4,4'-(1-PROPYL-1H-1,2,4-TRIAZOLE-3,5-DIYL)BIS(2,5-DIHYDRO-1,2,5-OXADIAZOL-3-AMINE) 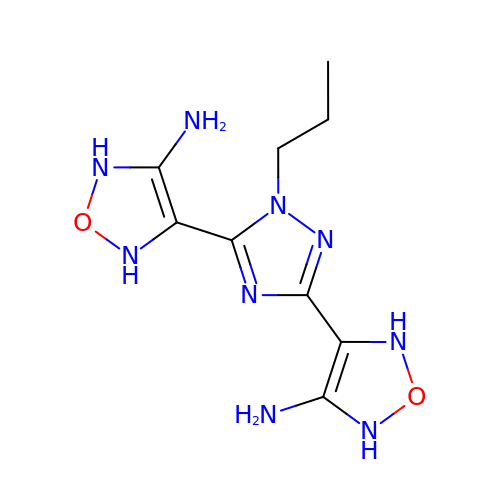| C9 H15 N9 O2 | AZHWQKVREXJRBF-UHFFFAOYSA-N>[2x]MASSAQDGNNPLFSPYKMGKFNLSHRVVLAPMTRCRALNNIPQAALGEYYEQRATAGGFLITEGTMISPTSAGFPHVPGIFTKEQVREWKKIVDVVHAKGAVIFCQLWHVGRASHEVYQPAGAAPISSTEKPISNRWRILMPDGTHGIYPKPRAIGTYEISQVVEDYRRSALNAIEAGFDGIEIHGAHGFLIDQFLKDGINDRTDEYGGSLANRCKFITQVVQAVVSAIGADRVGVRVSPAIDHLDAMDSNPLSLGLAVVERLNKIQLHSGSKLAYLHVTQPRYVAYGQTEAGRLGSEEEEARLMRTLRNAYQGTFICSGGYTRELGIEAVAQGDADLVSYGRLFISNPDLVMRIKLNAPLNKYNRKTFYTQDPVVGYTDYPFLQGNGSNGPLSRLLEHHHHHH

The biocatalytic reduction of the oxime moiety to the corresponding amine group has only recently been found to be a promiscuous activity of ene-reductases transforming α-oximo β-keto esters. By studying the crystal structures of enzyme oxime complexes, analyzing molecular dynamics simulations, and investigating biocatalytic cascades and possible intermediates, we obtained evidence that the reaction proceeds via an imine intermediate and not via the hydroxylamine intermediate. To gain more insight into the reaction pathway, we determined the crystal structures of the two enzymes OPR3 and XenA in complex with the oxime substrates 1a–c, either by co-crystallization or by soaking. All the crystal structures obtained had a high resolution (1.9–1.35 Å) and showed clear electron density features for the oximes.

To assess if the introduced amino acid exchanges affected the overall structure and the binding of the oxime, we also crystallized the tyrosine variants in complex with selected oxime substrates. The protomers in the crystal structures of the tyrosine variants are perfectly superimposable with the ones of the wild-type enzymes, confirming that the exchanges did not lead to major structural alterations. Interestingly, the binding mode of the oxime substrates also did not change in most of the structures. The propanoyl moiety of oxime 1b points into this cavity and is likely stabilized by hydrophobic interactions. Substrates with an acetyl moiety (such as oximes 1a and 1c) give the non-productive binding mode described above. Interestingly, the exchange of the canonical tyrosine (Y190F) did not have an observable effect in this experiment, indicating that fast protonation in the active site is feasible, likely via a water molecule. On the other hand, the canonical tyrosine variant OPR3_Y190F showed a 2-fold increase in kred and an 8-fold decrease for the NADPH Kd. Though a parallel 2-fold increase in kox is also observed, the Kd for the oxime seems not to be affected by the mutation, indicating that the canonical tyrosine residue does not play a role in substrate binding in this enzyme.>[14x]AEPVYPDQLRLFSLGQGVCGDKYRPVNREEAQSVKSNIVGMMGQWQISGLANGWVIMGPGYNGEIKPGTASNTWCYPTNPVTGEIPTLSALDIPDGDEVDVQWRLVHDSANFIKPTSYLAHYLGYAWVGGNHSQYVGEDMDVTRDGDGWVIRGNNDGGCDGYRCGDKTAIKVSNFAYNLDPDSFKHGDVTQSDRQLVKTVVGWAVNDSDTPQSGYDVTLRYDTATNWSKTNTYGLSEKVTTKNKFCWPLVGETELSICIAANQSWASQNGGSTTTSLSQSVRPTVPARSKIPVKIELYKADISYPYEFKADVSYDLTLSGFLRWGGNAWYTHPDNRPNWNHTFVIGPYKDKASSIRYQWDKRYIPGEVKWWDWNWTIQQNGLSTMQNNLARVLRPVRAGITGDFSAESQFAGNIEIGAPVPLAA

Aerolysin is a major contributor to the pathogenicity of Aeromonas spp, which causes gastroenteritis, deep wound infections and sepsis in humans. It is a pore-forming toxin (PFT), which is secreted by the bacterium as a water-soluble protein, binds receptors on their target cell membrane and, following proteolytic activation, forms circular heptameric oligomers that insert into the plasma membrane thus permeabilizing it, potentially leading to cell death. Aerolysin belongs to the family of β-PFTs, meaning that the final pore spans the membrane in the form of a β-barrel and defines the aerolysin-like family of proteins that share a common structural motif3. Combined, these structures, consistent with the recent lysenin pore structure, describe the major steps involved in the pore-formation process by aerolysin: the transition from the monomer to the oligomer with the formation of two highly stable concentric β-barrels, the zipper-like formation of the β-barrel and the final piston-like puncturing of the lipid bilayer.

We next analysed the structure of a second aerolysin mutant (K246C/E258C). While the Y221G mutation, which is positioned just two amino acids downstream of the inner β-barrel (star in Fig. 1e), prevents the prestem loop from moving away from the five-stranded sheet in domain 3, the second mutant leads to a block at later stages, namely, hindering the formation of the full transmembrane β-barrel. Due probably to stochastic difference in kinetics and steric constraints, only one of the heptamers is able to undergo quasipore formation with extension of the inner β-barrel, leaving just enough space for the second heptamer in the dimer to undergo progression to the post-prepore state. The resolution of the obtained EM map is 4.5 Å and locally extends from 3.5 to 4.5 Å. The density corresponding to the prestem loop partially disappears from the pocket between the subunits, as it becomes unstructured and flexible. The transition from the post-prepore to the quasipore state involves two major conformational rearrangements of the protein. First, the inner β-barrel, which will eventually form the transmembrane pore, elongates by incorporating 15 more residues from the prestem loop (c shown in yellow). Second, the protein undergoes a vertical collapse, which translates the extended inner β-barrel and the outer β-barrel 39 Å towards the target membrane.> MALINPQFP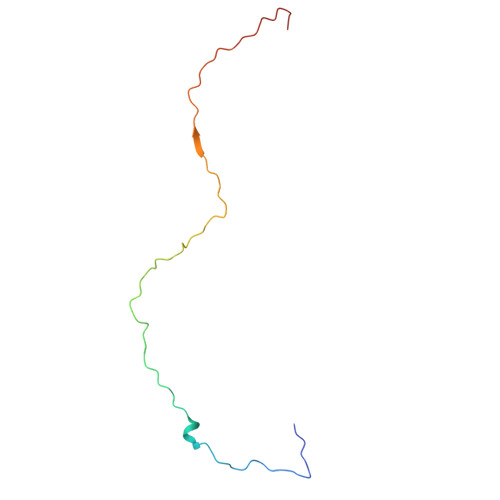YAGPVPIPGPAPTETMPLLNYRVEGRIAGIQQARQFMPFLQGPHREVAEQTYYAIGTGIQMGQTFNQPLINTQEG>[2x]MKLDIKKTFSNRSDRVKGIDFHPTEPWVLTTLYSGRVELWNYETQVEVRSIQVTETPVRAGKFIARKNWIIVGSDDFRIRVFNYNTGEKVVDFEAHPDYIRSIAVHPTKPYVLSGSDDLTVKLWNWENNWALEQTFEGHEHFVMCVAFNPKDPSTFASGCLDRTVKVWSLGQSTPNFTLTT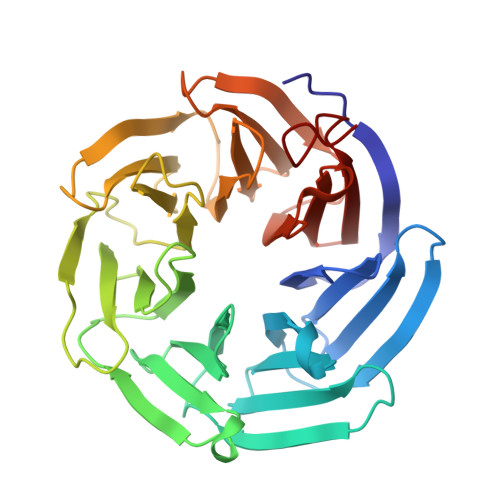GQERGVNYVDYYPLPDKPYMITASDDLTIKIWDYQTKSCVATLEGHMSNVSFAVFHPTLPIIISGSEDGTLKIWNSSTYKVEKTLNVGLERSWCIATHPTGRKNYIASGFDNGFTVLSLGNDEHHHHHH>UGIGGU[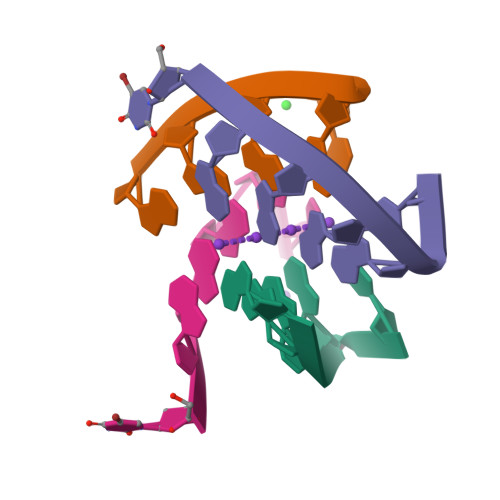8x]>QDSTSDLIPAPPLSKVPLQQNFQDNQFHGKWYVVGKAGNHDLREDKDPRKMQATIYELKEDKSYNVTNVRFVHKKCNYRIWTFVPGSQPGEFTLGNIKSWPGLTSWLVRVVSTNYNQHAMVFFKRVYQNRELFEITLYGRTKELTNELKENFIRFSKSLGLPENHIVFPVPIDQCIDGSAWSHPQFEK[2x];>[2x]MPLSPPTNLHLEANPDTGVLTVSWERSTTPDITGYRITTTPTNGQQGNSLEEVVHADQSSCTFDNLSPGLEYNVSVYTVKDDKESVPISDTIIPEVPQLTDLSFVDITDSSIGLRWTPLNSSTIIGYRITVVAAGEGIPIFEDFVDSSVGYYTVTGLEPGIDYDISVITLINGGESAPTTLTQQTAVPPPTDLRFTNIGPDTMRVTWAPPPSIDLTNFLVRYSPVKNEEDVAELSISPSDNAVVLTNLLPGTEYVVSVS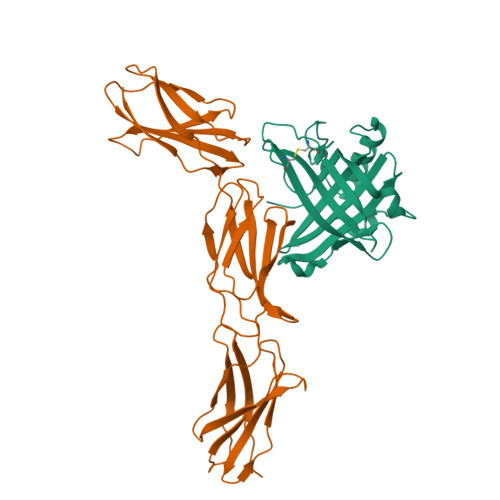SVYEQHESTPLRGRQKTGSAHHHHHH>[6x]GQDCTFFFPQTEGTVWVRKGYDAKGNLQSVMSYQVDEVETLPSGQEVEADYVYTNPSGTIVNKGDIKAYCQNGEFFLDSKETLSYPGVV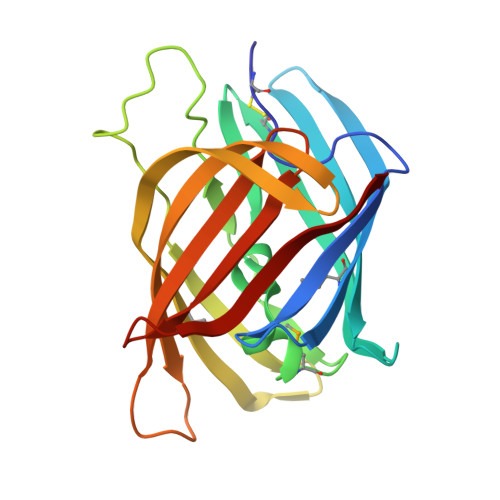SEMNTNVDITENFINYPNPYAANFDKNNVYFDEASVKIYDKKNRKNRKDMAIKDREFIKTESITTPAGTFDCAKVKYNIATRSPKSKETITGYGYEWYSPNVGLVRTEQYDKNNVLQSYTVLEELK Botulinum neurotoxins (BoNTs), secreted by neurotoxigenic Gram-positive strains of Clostridia, are the most toxic bacterial proteins known. Each BoNT is synthesized as a large precursor that is cleaved into two polypeptide chains that remain connected through an interchain disulfide bond: a heavy chain (HC, ∼100 kDa) and a light chain (LC, ∼50 kDa). The LC domain is a zinc-dependent protease that cleaves components of the soluble N-ethylmaleimide-sensitive-factor attachment receptor (SNARE) family of proteins, a process that blocks acetylcholine release at the neuromuscular junction and thereby causes flaccid paralysis of muscles. BoNT/A and E cleave synaptosomal-associated protein 25 (SNAP-25) and BoNTs B, D, F, and G cut vesicle-associated membrane protein (VAMP).

Catalytically inactive recombinant LC/A3 spanning residues Pro2–Lys417 and containing the double mutation Glu224Gln/Phe336Tyr was produced with an N-terminal cleavable 6xHis tag by bacterial expression (for details, see experimental procedures). Crystals suitable for the determination of the high-resolution structure of LC/A3 grew within 1–2 weeks, diffracted to 2.0 Å resolution and belong to the space group P212121, with two molecules per asymmetric unit. The LC/A3 structure represents the typical globular BoNT-LC domain fold with a conserved groove that extends from the catalytic site around the enzyme. The electron density is well defined for all residues, with the exception of loop 200 (amino acid residues Ser201-Ala212 and Glu203-Ala203 of chain A and B, respectively), which is likely to be disordered. BoNT/A3 is the subtype with the least conserved LC among subtypes and shares 81.9% sequence identity with LC/A1. The overall structural organization of the LPH region, however, is conserved between LC/A1 and LC/A3. Our structure also confirms the observation of Pellett et al. that the LPH region in LC/A3 contains a cluster of basic amino acids that is absent in LC/A1 (20). In our structure loop 250 has a different conformation and points away from the active site. This different orientation of loop 250 may explain the inability of LC/A3 to undergo autocleavage. However, the observation that their catalytic pockets are virtually identical and other substrate-binding residues are largely conserved suggests that LC/A3 may accommodate SNAP-25 in a similar way as LC/A1.

>[2x]GSMPFVNKQFNYRDPVNGVDIAYIKIPNAGQMQPVKAFKIHEGVWVIPERDTFTNPEEGDLNPPPEAKQVPVSYYDSTYLSTDNEKDNYLKGVIKLFDRIYSTGLGRMLLSFIVKGIPFWGGSTIDTELKVIDTNCINVIEPGGSYRSEELNLVITGPSADIIQFECKSFGHDVFNLTRNGYGSTQYIRFSPDFTFGFEESLEVDTNPLLGAGTFATDPAVTLAHQLIHAAHRLYGIAINPNRVLKVKTNAYYEMSGLEVSFEELRTFGGNDTNFIDSLWQKKFSRDAYDNLQNIARILNEAKTIVGTTTPLQYMKNIFIRKYFLSEDASGKISVNKAAFKEFYRVLTRGFTELEFVNPFKVINRKTFLNFDKAVFRINIVPDENYTINEGFNLEGANSNGQNTEINSRNFTRLKNFTG>[2x]GSLTSDLGKQIKLKEVEGTLLQPATVDNWSQIQSFEAKPDDLLICTYPKAGTTWIQEIVDMIEQNGDVEKCQRAIIQHRHPFIEWARPPQPSGVEKAKAMPSPRILKTHLSTQLLPPSFWENNCKFLYVARNAKDCMVSYYHFQRMNHMLPDPGTWEEYFETFINGKVVW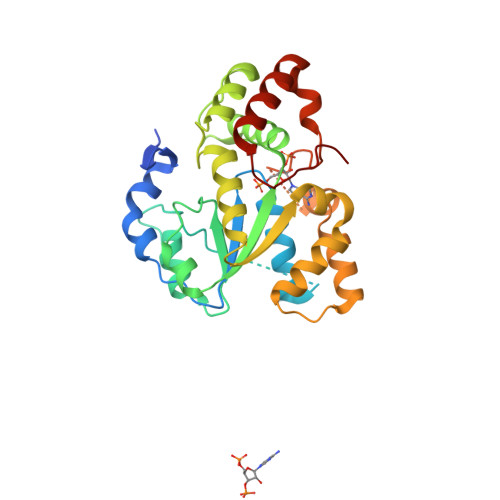GSWFDHVKGWWEMKDRHQILFLFYEDIKRDPKHEIRKVMQFMGKKVDETVLDKIVQETSFEKMKENPMTNRSTVSKSILDQSISSFMRKGTVGDWKNHFTVAQNERFDEIYRRKMEGTSINFSMEL>[2x]ASAPILIQGAMDVEVETLVAALKDKQELTVGSWTYWQGTLSGYPVVVSRTEVGLANAAAATTLAMERFQPRLVINQGTAGGHDPALHRGDIVIGTKSFNMGAYRSDLTPAEQGVDPSKWH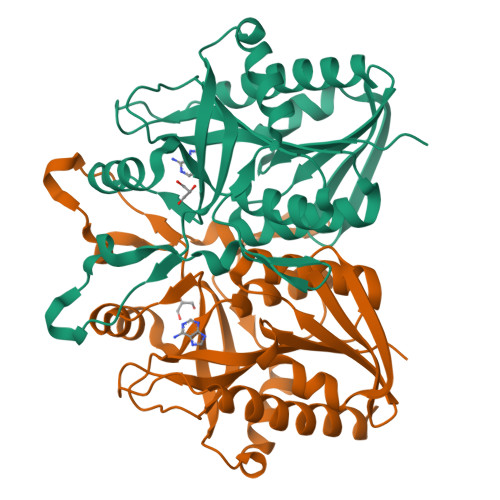NFEVTMRLRDNGKLVEHSSFAGDPELVGRALGMADRYRHGRVVPGIIGTADEWNRQVARINWLHQTYQTAAEEMETSSAALVAEAYKVPFVGIRVLSNTDLHGEEFDPQTAIHCQQFVIDYAKALINGF Research on IMP3 largely focused on its association with many cancer-related tumor entities, since its re-expression correlates with a poor prognosis for patients, classifying IMP3 as a tumor marker. Importantly, we used a very long degenerate sequence (N40) as a basis for SELEX, to allow multiple RNA contacts with more than a single RNA-binding domain, and a corresponding bioinformatic spacing analysis. This led us to the discovery that IMP3 recognizes—through the activity of all of its tandem RNA-binding domains—an extended array of multiple cis-acting RNA elements, composed of CA-rich motifs and sequences with a common GGC core. Members of the IMP protein family are prime examples for multidomain RBPs, where both affinity and specificity are achieved through simultaneous engagement of multiple domains with their respective RNA elements. Taken together, our in-depth analysis of sequence requirements for IMP3–RNA interaction and the functional validation supports the suggested safe-housing mechanism: Through sequence-specific formation of RNP complexes, IMP3 shields a specific region within the HMGA2 3′-UTR that contains miRNA-binding sites in close proximity, thereby protecting the mRNA from let-7-mediated repression.

Our SELEX approach based on a N40-degenerate sequence revealed that the KH domains recognize two different types of RNA motifs: CA-rich motifs and elements with a common GGC core. To determine the individual contributions of KH1 and 2 (Lys192 to Ile355), their RNA binding was inactivated by mutation (GKEG motif to GDDG), while maintaining the crucial tandem context, resulting in four possible combinations. Our NMR data clearly proved the integrity of all constructs. SAXS (small-angle X-ray scattering) data back-calculated based on the crystal structure are in good agreement, indicating that the crystal structure reflects the monomeric solution geometry, which also closely resembles other tandem KH domains. Indeed, KH1 clearly favors binding of the GGC motif, while KH2 prefers binding to the CA-RNA. Given that larger NMR CSPs were observed for the KH1/GGC, compared with the KH2/CA-RNA interaction, RNA binding appears to be mediated primarily through KH1. Indeed, ITC revealed a measurable KH1–GGC interaction in the low-to-medium micromolar range, while the KH2–CA complex could not be determined in our ITC setup. As expected, a 10-fold higher affinity compared with the single interactions of 7-mer RNAs indicates a cooperative binding event that shifts affinity by one order of magnitude. Our data suggest that in complex with KH1–2—similar to the situation with KH3–4— the RNA adopts a looped conformation that fits the narrow window for linker length between motifs.

> GAMAKPCDLPLRLLVPTQFVGAIIGKEGATIRNITKQTQSKIDVHRKENAGAAEKSITILSTPEGTSAACKSILEIMHKEAQDIKFTEEIPLKILAHNNFVGRLIGDDGRNLKKIEQDTDTKITISPLQELTLYNPERTITVKGNVETCAKAEEEIMKKIRESYENDI> MVHGKLKEAAEVTGSVSLEALEEVQVGENIEVGVGIDELVNAEAFAYDFTLNYDENAFEYVEAISDDGVFVNAKKIEDGKVRVLVSSLTGEPLPAKEVLAKVVLRAEAKTEGSNLSVTNSSVGDGEGLVHEIAGTEKTVNIIEGTSPEIVVNPVRDFKASEINKKNVTVTWTEPETTEGLEGYILYKDGKKVAEIGKDETSYT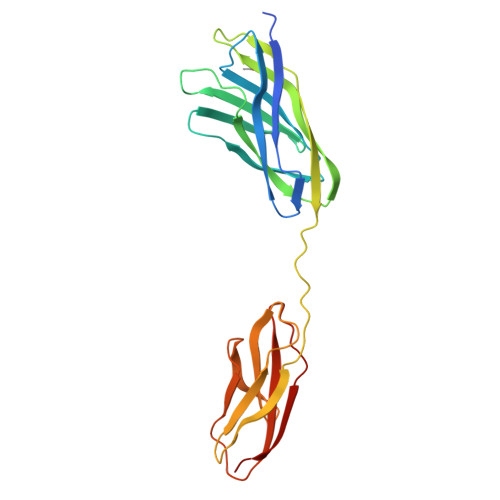FKKLNRHTIYNFKIAAKYSNGEVSSKESLTLRTAR> MAVPQFHRPSTVTTDSVRALGMRGLVLATNNSQFIMDNNHPHPQGTQGAVREFLRGQAAALTDLGLAHANNTFTPQPMFAGDAPA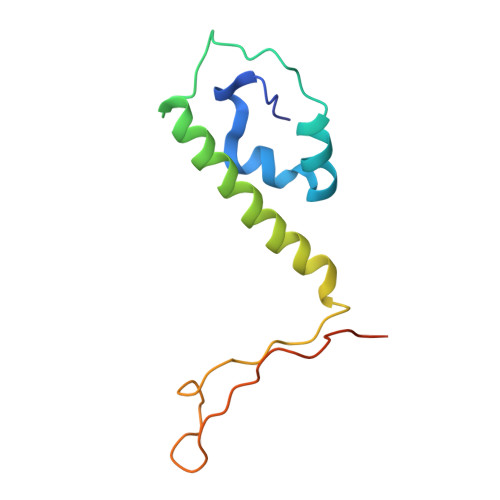AWLRPAFGLRRTYSPFVVREPSTPGTP> NSSSLNVDGRSSKQHGKRDSKITDHFVRIPKSEDKRKEQCEVRHQRAERKIPKYVPPNLPPDKKWLGTPIEEMRKMPRCGVRLPLLRPSASHTVTVRVDLLRAGEVPKPFPTHYKDLWDNKHVKMPCSEQNLYPVEDENGERTAGSRWELIQTALLNKFTRPQNLKDAILKYNVAYSKKWDFTALVDFWDKVLEEAEAQHLYQSILPDMVKIALCLPNICTQPIPLLKQKMNHSVTMSQEQIASLLANAFFCTFPRRNAKMKSEYSSYPDINFNRLFEGRSSRKPEKLKTLFCYFRRVTEKKPTGLVTFTRQSLEDFPEWERC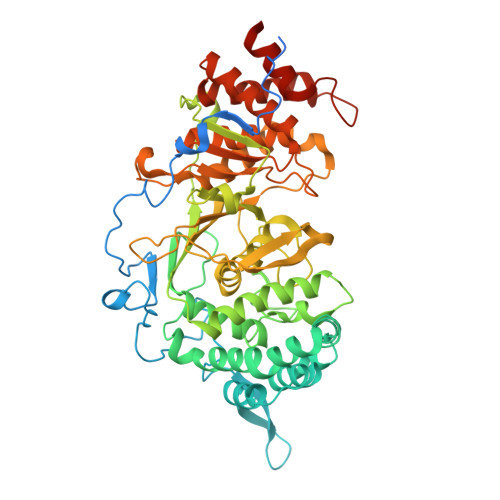DKPLTRLHVTYEGTIEGNGRGMLQVDFANRFVGGGVTGAGLVQEEIRFLINPELIVSRLFTEVLDHNECLIITGTEQYSEYTGYAETYRWARSHEDGSEKDDWQRCCTEIVAIDALHFRRYLDQFVPEKVRRELNKAYCGFLRPGVPPENLSAVATGNWGCGAFGGDARLKALIQLLAAAAAERDVVYFTFGDSELMRDIYSMHTFLTERKLNVGKVYRLLLRYYREECRDCSSPGPDTKLYPFIYHAAESSAETSDQPGQRTGT>[2x]MAHHHHHHVDDDDKMVHHDGFQTVKATIDWEHPMFKLYEKAKRNGKWNPADIDFSQDQKDFASLTSEEKISALPLVAGFSAGEEAVTLDILPMAHALARQGRLEDVLFLTTFMHDEAKHVE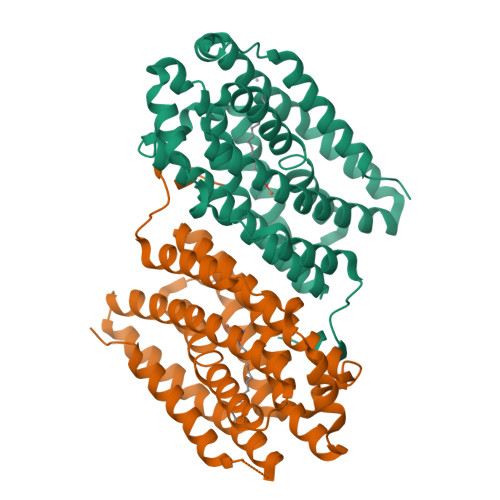MFSRWQQAVGIGQMDLSVFHNDHYKRIFYEALPEAMNRLYADDSPEAVIRAATVFNMIVEGTLAESGYYTFRQIYKKAGLFPGLLQGIDYLNMDEGRHIQFGIYTIQRIVNEDERYYELFIRYMDELWPHVIGYVDYLTELGKRQQQLARTYALEIDYDLLRHYVIKQFNLRKKQISRTKRVDVVEGLEKTAAES> MARSNLLRDKKV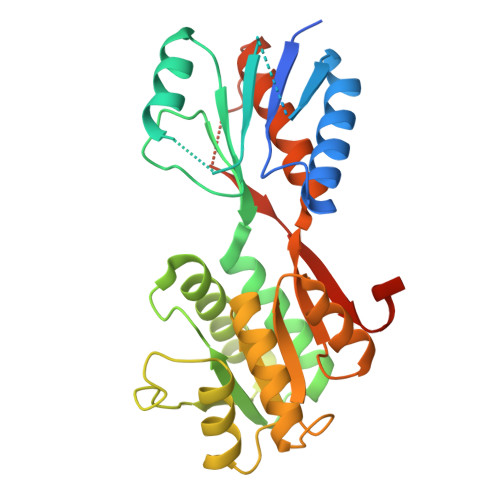EKEPIKPKIVLISHIKTNPYWLDIKAGAERAAKERGAVVEFLGPTTASTEDGLKLFDMATSAKVSGIITYVQEEGQYKKKINSAMEKGIPVVTIASDEEDSNRIAYVGTDNVLAGQVAGKEMVKQIGTSGNVAIVMGGKNVKNQKERVEGFTQYIKSNSNLKIVDTDSSDAMLLEAEIITRKILNRNDNINALFCTSALDGIGAARAVKDLNYKDRVKIICFDDLDDTLSNIRNGLVSATIVQKSNEMGYRAVNIIMDKIEGKSNKFSKSLIDVNVINKSDVDSYKRGDDKVEN>MSILFSSILFSIATFFSRILGLFRDVLFAKYFGVSYELDAYFIAIMFPFFLRKVFGEGAMSSAFVPLYSEKSGEEKDKFLSSVINGFSLIILALVILSYFFPELIINLFGAGSSHETKILAKKLLLITSPSIYFIFLWAISYSILNTNNKFFWPALTPSISNITIIIGTFLSTKYGIISPTIGFLIGSILMFFSIIKSIIKHKYYFTIKHFPHFLKLFFPTFMTMVVSQINTVVDMNVVSFYDKGSISYLQYASRFYLLPYGLFAVSVSTVVLSKISNDRKNFNYHLNDALKTTLFFTIPSMVGLIFLSTPIIRFFYEHGAFTSKDTLITSKILIAYTLGLPFYGIYSTISRSYHAIKNTKTPFIAATIVSLSNIILDIIFGLKYGPIGVALATSIAGIIGVLYLLFSVKTFPIKDFLKISLNSLIMLFVIYLTDFTDNEFWFLIQILIGILVYLIFSSIFYRDLIRRFLYARKK[2x]

The cytoplasmic-facing Lipid II is flipped to the periplasmic side of the membrane by a Lipid II flippase, after which the GlcNAc-MurNAc-pentapeptide moiety is incorporated into peptidoglycan and the lipid carrier is recycled. MurJ consists of 14 transmembrane helices (TMs), of which the first 12 are organized into two 6-TM bundles termed the N-lobe (TMs 1–6) and C-lobe (TMs 7–12). The N-lobe and C-lobe enclose a central cavity that is large and highly cationic, properties consistent with Lipid II transport. We determined four crystal structures of MurJTA: one structure in an outward-facing conformation to 1.8 Å resolution, and three structures in inward-facing conformations distinct from the published structure, resolved to 3.2, 3.0, and 2.6 Å, respectively.

Based on the conformation at these regions and the size of the membrane portal, we assigned two of the structures as inward-closed and inward-open. The Cα-Cα distance between Ser11 (TM 1) and Ser267 (TM 8) increased from 8.0 Å in the closed structure to 17.4 Å in the open structure. Superposition of all the inward-facing structures show that they align well at the periplasmic end of the protein, which highlights the importance of the periplasmic gate in stabilizing the inward-facing state. We observed systematic rearrangement of Arg24, Asp25, and Arg255 (Arg270 in MurJEC) in the cavity between the different crystal structures. In light of this discovery, we re-analyzed the Na+ site in all our other MurJ structures and found electron density in the inward-occluded and inward-closed structures as well, albeit much weaker. Because of the high concentration of Na+ in the crystal drop outweighing the potentially lower Na+ affinity in the inward-facing state, we posit that these weak densities would correspond to Na+, possibly reflecting the inward-facing pre-Na+-release conformation of MurJ.> TTI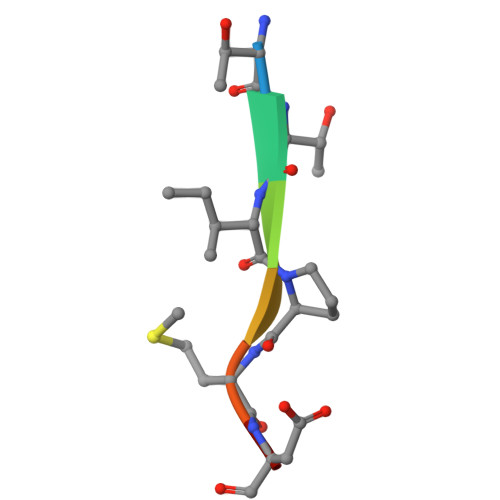PMDS> ISLGELGLLPSTVLAIGYYENFVSTVCDALHSLPTIKLNGIEYKDFVFNIIIPNDLDADIKRRAQIYFKKMDIHEVKIDTNGRSFPLYLQIDEENSGDVAVLYDMPTTLGGIDKAIEMYMKKGHIGKTSQQQLLEERELRNFKTTLINLIN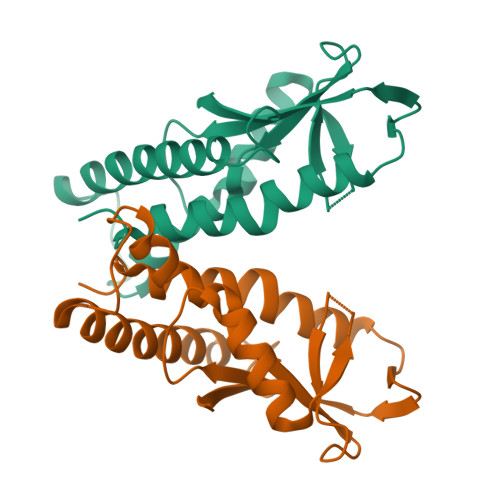NNSFTKTFVKVIEE> GKEKLPKMRLPTRSDMIC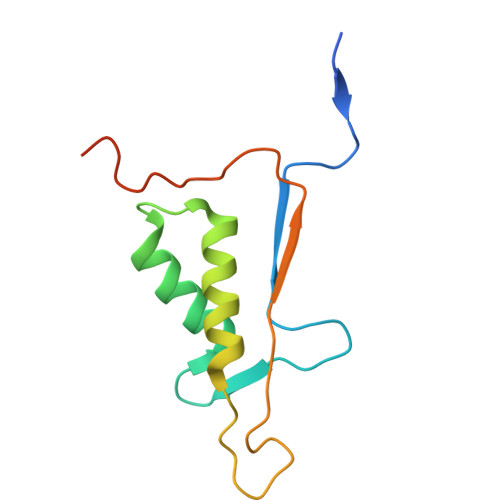GYACLKGTAAMRNAKRGSWYIEALAQVFSERACDMHVADMLVKVNALIKDREGYAPGTEFHRCKEMSEYCSTLCRHLYLFPGHPPTLEHHHHHH> GAMGSKPDTHRADERRFLDERGSSGPLAPNGLNPATIMEKAVRERIVESYFWKEQCFGVNEADIVDRVVEHVRFVGGVTGVTQKPSPFLCLAFKLLQLAPGDDILKEYLYFGGEKFKYLRALAAFYIRLTRPDKEVYTLLEPFLEDRRKLRRKGKNGTSLTYMDEFIDDLLTKDRVCSTSLWKMRRRDILEDLDLLEPRVSPLGSLEDILEEEEQAAKNED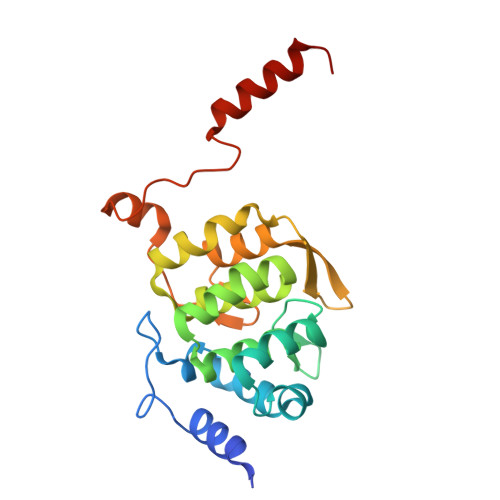GE In this work, we exhaustively probe the ability of all 36 immobile HJ sequences to form DNA crystals in two different designed systems. Three separate self-assembling DNA crystal systems are described in this report: the “4 × 5” and “4 × 6” designs (collectively referred to as the 4 × N systems), and a third construct with a “scrambled” sequence variant of the 4 × 6 lattices. Self-assembly was mediated by three constituent oligonucleotides: (S1) containing four sequence repeats of either 5 or 6 bases; (S2) composed of 21 bases containing complementary regions to both (S1); and (S3) which forms the second junction crossover. The HJ serves as the fundamental component at the core of each unit, and the ultimate assembly of the full lattice is facilitated by the complementary 2-base sticky ends that tail each duplex.

Each asymmetric unit could be defined as either a HJ containing 10 and 11 bp on each arm, or as a 21-bp linear duplex. Both versions were solved in parallel, yielding a total of 134 crystal structures (Supplementary Table 1 for data collection and refinement statistics). The 4 × 5 system robustly crystallized with 75% of the junctions, and we obtained crystals in all but 9 of 36 sequences. Of the resulting structures, 18 exhibited P32 symmetry with average cell dimensions a = b = 68.85 Å c = 60.09 Å, with only nine retaining the original P3221 symmetry with average cell edges a = b = 68.17 Å c = 60.60 Å. Although the cell parameters between the two symmetries were virtually indistinguishable, the differences between the periodicity of the lattices is dramatic, with vastly different cavity sizes. Although in the majority of cases, the individual junctions, regardless of design parameters, had a preference for crystallizing in cacodylic acid within the 6.0–6.5 pH regime, not all crystals were confined to this requirement. Pos1 and 2 were readily observable in the electron density maps at either one or both of these conserved sites in a significant number of the structures, with no apparent respect to motif or symmetry.

> GAGCAGACGTG;> ACACCACTCA;> CATGT;> TCTGAGTGGCGTCTGC(3S)-N7,3-dimethyl-N5-[(1R,5S)-3-oxabicyclo[3.1.0]hexan-6-yl]-3-phenyl-2H-1-benzofuran-5,7-dicarboxamide 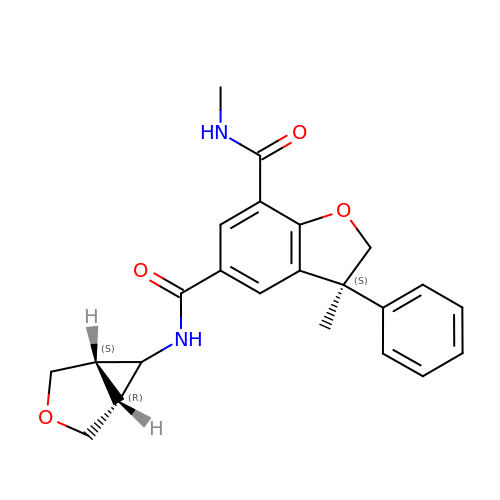| C23 H24 N2 O4 | RDGLEZJKVBSRJX-MUCNXURCSA-N>MSQHINTVGYLEQKMFAAMVA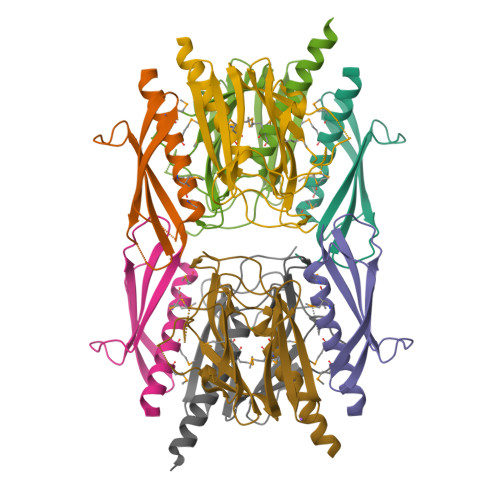DNQMAMVMLNPKNLKASNGEEELAGQTWYWKVAPVATTQPLLKAFDVSVAATTQASPIITVRSYVASENLYFQGGGHHHHHH[4x];>[4x]MNQVQRSNELSQERTARLNELQRALVMMDSDFRQIALRQTRTNGEEPSKKLLHWADYLLDSDNKGIMFARLGWHNPQQQFPRGEVTKVGYRIKDERLERVWWRYPDTPAGQEGVVTPLLSDVEELNVRFYDGKQWINEWSNELTLPAAISVELTLKDYGKIARTYLTPEGNLQKQ>[2x]GSHMKPECVQQLLVCSQEAKQSAYCPYSHFPVGAALLTQEGRIF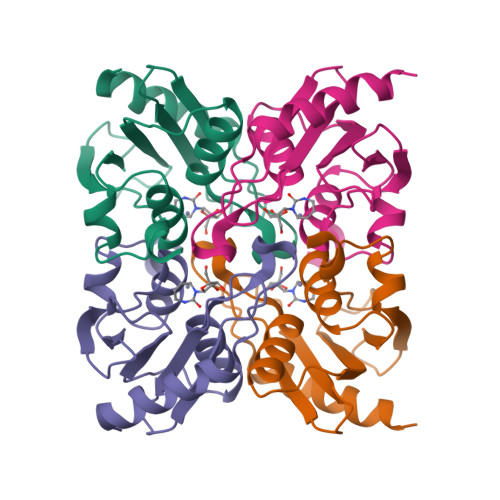KGCNIENACYPLGICAERTAIQKAVSEGYKDFRAIAIASDMQDDFISPCGACRQVMREFGTNWPVYMTKPDGTYIVMTVQELLPSSFGPEDLQKTQ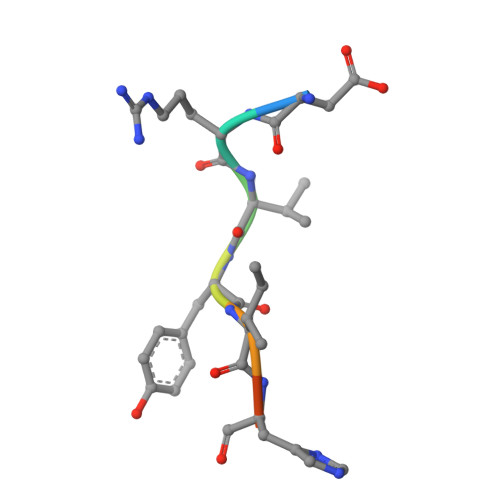> DRVYIHPF> SNASRLVTTPQKR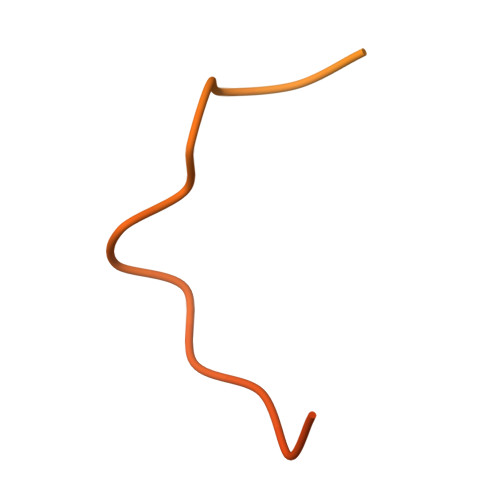AYGFSFSAYGSPTSPSSSASSTPGAFGQSILSSSINRGLNKSISASNLRRSLNVEDSILQPGAFSANSSMRLLGGPGSHKK>GSHMSGRVGDLSPRQKEALAKFRENVQDVLPALPNPDDYFLLRWLRARSFDLQKSEAMLRKHVEFRKQKDIDNIISWQPPEVIQQYLSGGMCGYDLDGCPVWYDIIGPLDAKGLLFSAS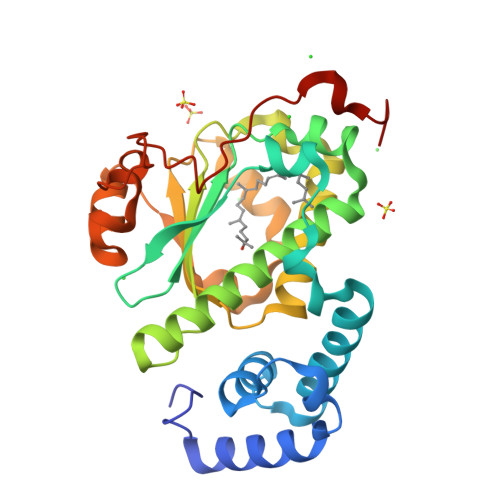KQDLLRTKMRECELLLQECAHQTTKLGRKVETITIIYDCEGLGLKHLWKPAVEAYGEFLCMFEENYPETLKRLFVVKAPKLFPVAYNLIKPFLSEDTRKKIMVLGANWKEVLLKHISPDQVPVEYGGTMTDPDGNPKCKSKINYGGDIPRKYYVRDQVK[2x]>[6x]MDSFNPTTKTQAALTAALQAASTAGNPEIRPAHLLMALLTQNDGIAAPLLEAVGVEPATVRA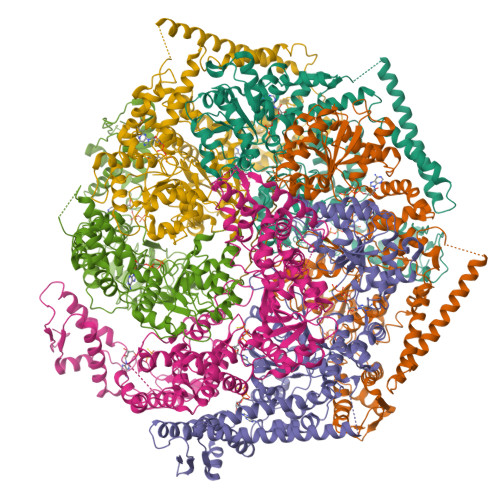ETQRLLDRLPQATGASTQPQLSRESLAAITTAQQLATELDDEYVSTEHVMVGLATGDSDVAKLLTGHGASPQALREAFVKVRGSARVTSPEPEATYQALQKYSTDLTARAREGKLDPVIGRDNEIRRVVQVLSRRTKNNPVLIGEPGVGKTAIVEGLAQRIVAGDVPESLRDKTIVALDLGSMVAGSKYRGEFEERLKAVLDDIKNSAGQIITFIDELHTIVGAGATGEGAMDAGNMIKPMLARGELRLVGATTLDEYRKHIEKDAALERRFQQVYVGEPSVEDTIGILRGLKDRYEVHHGVRITDSALVAAATLSDRYITARFLPDKAIDLVDEAASRLRMEIDSRPVEIDEVERLVRRLEIEEMALSKEEDEASAERLAKLRSELADQKEKLAELTTRWQNEKNAIEIVRDLKEQLEALRGESERAERDGDLAKAAELRYGRIPEVEKKLDAALPQAQAREQVMLKEEVGPDDIADVVSAWTGIPAGRLLEGETAKLLRMEDELGKRVIGQKAAVTAVSDAVRRSRAGVSDPNRPTGAFMFLGPTGVGKTELAKALADFLFDDERAMVRIDMSEYGEKHTVARLIGAPPGYVGYEAGGQLTEAVRRRPYTVVLFDEIEKAHPDVFDVLLQVLDEGRLTDGHGRTVDFRNTILILTSNLGSGGSAEQVLAAVRATFKPEFINRLDDVLIFEGLNPEELVRIVDIQLAQLGKRLAQRRLQLQVSLPAKRWLAQRGFDPVYGARPLRRLVQQAIGDQLAKMLLAGQVHDGDTVPVNVSPDADSLILG> HPETLVKVKDAEDQLGARVGYIELDLNSGKILESFRPEERFPMMSTFKVLLCGAVLSRVDAGQEQLGRRIHYSQNDLVEYSPVTEKHLTDGMTVRELCSAAITMSDNTAANLLLTTIGGPKELTAFLHNMGDHVTRLDRWEPELNEAIPNDERDTTMPAAMATTLRKLLTGELLTLASRQQLIDWMEADKVAGPLLRSALPAGWFIADKAGAGERGSRGIIAALGP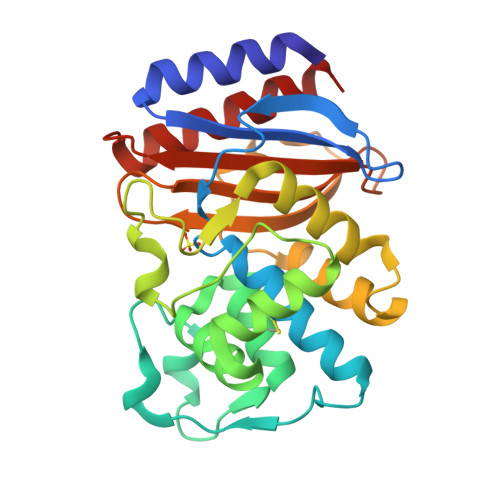DGKPSRIVVIYTTGSQATMDERNRQIAEIGASLIKHW>[2x]PSVYDAAAQLTADVKKDLRDSWKVIGSDKKGNGVALMTTLFADNQ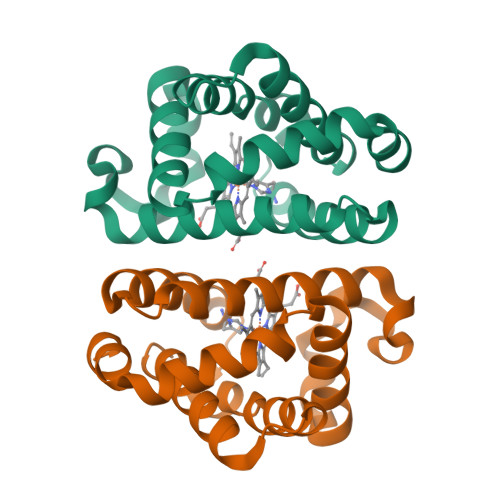ETIGYFKRLGDVSQGMANDKLRGHSIALMYALQNFIDQLDNPDDLVCVVEKFAVNHITRKISAAEFGKINGPIKKVLASKNFGDKYANAWAKLVAVVQAAL> DLLELTEDMEKEISNALG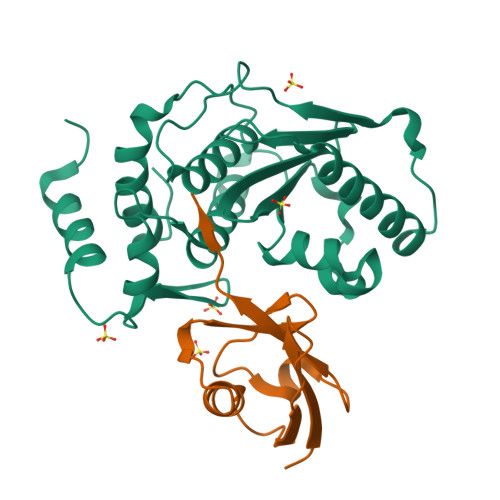HGPQDEILSSAFKLRITRGDIQTLKNYHWLNDEVINFYMNLLVERNKKQGYPALHVFSTFFYPKLKSGGYQAVKRWTKGVNLFEQEIILVPIHRKVHWSLVVIDLRKKCLKYLDSMGQKGHRICEILLQYLQDESKTKRNSDLNLLEWTHHSMKPHEIPQQLNGSDCGMFTCKYADYISRDKPITFTQHQMPLFRKKMVWEILHQQLL;> EGEYIKLKVIGQDSSEIHFKVKMTTHLKKLKESYCQRQGVPMNSLRFLFEGQRIADNHTPKELGMEEEDVIEVYQEQTGG> ETGAHPPEIIRKPQNQGVRVGGVASFYCAARGDPPPSIVWRKNGKKVSGTQSRYTVLEQPGGISILRIEPVRAGRDDAPYECVAENGVGDAVSADATLTIY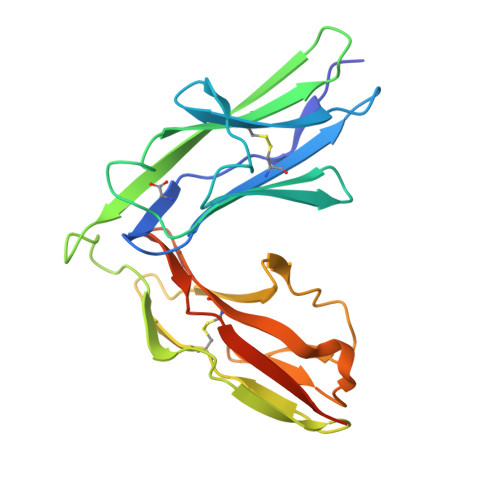EGDKTPAGFPVITQGPGTRVIEVGHTVLMTCKAIGNPTPNIYWIKNQTKVDMSNPRYSLKDGFLQIENSREEDQGKYECVAENSMGTEHSKATNLYVKVRRVGTKHHHHHH> MNKVIVAAFVSAFVLGSTA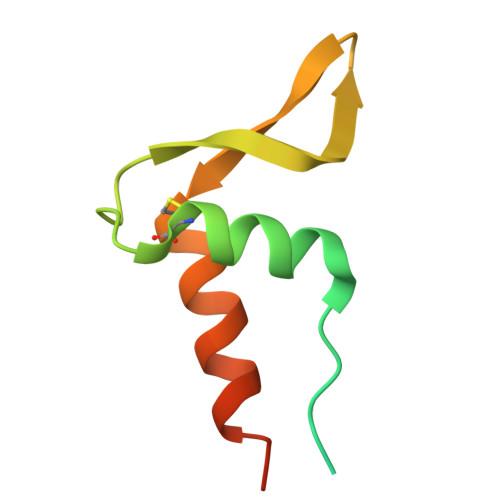TFASGNLESSLAPISAKDMLDYLACKDKKPTDVVKSHTEVENGKIVRVKCGDIVALVQKAREQSGDAWQGGY>MDLEEQKKAVIEKLIREGYIKSKRVIDALLKVPREEFLPEHLKEYAYVDTPLEIGYGQTISAIHMVGMMCELLDLKPGMKVLEIGTGCGYHAAVTAEIVGEDGLVVSIERIPELAEKAERTLRKLGYDNVIVIVGDGTLGYEPLAPYDRIYTTAAGPKIPEPLIRQLKDGGKLLMPVGRYLQRLVLAE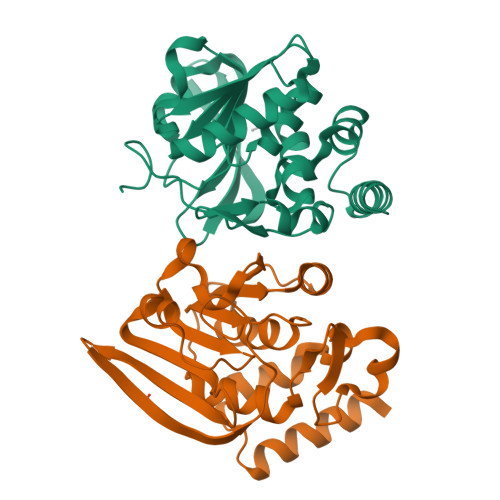KRGDEIIIKDCGPVAFVPLVGKEGFQG[2x]>[6x]MRIEKWVVREHLDGVPDVNRVYEKVVEDVRIDLRPDEMLFRTRYVSVDPYQNGLALETPIGHHMGADSIMEVVEAGPAAAFAVGDLVQGFGGWR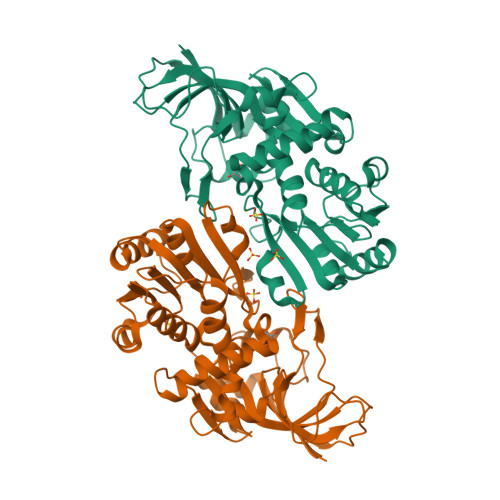THVVHNGAEELWTTGIFPMVFPAYRRLDPSWYGERLPVSTALGIMGAPGMTAWGTLTRFLEVRPGDTVVVSGASGSIGTLVGQLAKRAGAGRVVGTTGSPGKAEYLRELGFDEVVLYTQGDDAEKVRQALLLAAPDGVDRYFDNLGGTVTDAVFTMLNVDSRVAVCWQWATTVNGELTGPRLLPYIMFPRTTIRGIFAQEWFTEPLLAQMHQELGGLVRDGEIRYHQTVHKGFDEIPAAYRSLYLDREHNRGKVLVEV> MASIDAFSDLERRMDGFQKDVAQVLARQQNHVALYERLLQLRVLPGASDVHDVRFVFGDDSRCWIEVAMHGDHVIGNS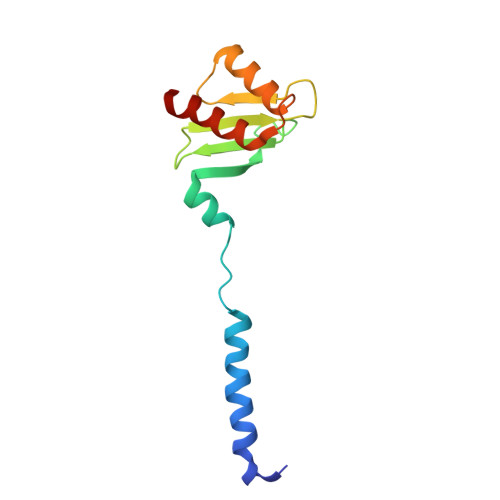HPALDPKSRATLEHVLTVQGDLAAFLVVARDMLLASL>MANSGCKDVTGPDEESFLYFAYGSNLLTERIHLRNPSAAFFCVARLQDFKLDFGNSQGKTSQTWHGGIATIFQSPGDEVWGVVWKMNKSNLNSLDEQAGVKSGMYVVIEVKVATQEGKEITCRSYLMTNYESAPPSPQYKKIICMGAKENGLPLEY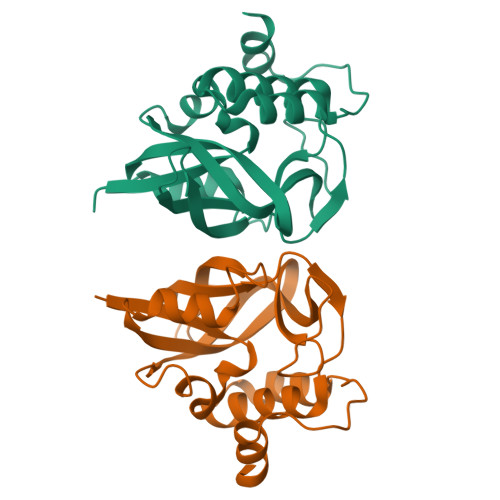QEKLKAIEPNDYTGKVSEEIEDIIKKGETQTL[2x]>MRCVGVGNRDFVEGLSGATWVDVVLEHGGCVTTMAKNKPTLDIELQKTEATQLATLRKLCIEGKITNITTDSRCPTQGEAILPEEQDQNYVCKHTYVDRGWGNGCGLFGKGSLVTCAKFQCLESIEGKVVQHENLKYTVIITVHTGDQHQVGNETQGVTAEITSQASTAEAILPEYGTLGLECSPRTGLDFNEMILLTMKNKAWMVHRQWFFDLPLPWTSGATTKTPTWNRKELLVTFKNAHAKKQEVVVLGSQEGAMHTALTGATEIQTSGGTSIFAGHLKCRLKMDKLKLKGMSYAMCLNTFVLKKEVSETQHGTILIKVEYKGEDAPCKIPFSTEDGQGKAHNGRLITANPVVTKKEEPVNIEAEPPFGESNIVIGIGD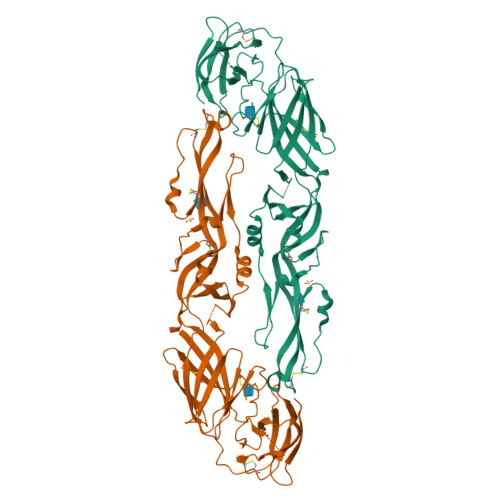KALKINWYRKGF[3x]>MSSEY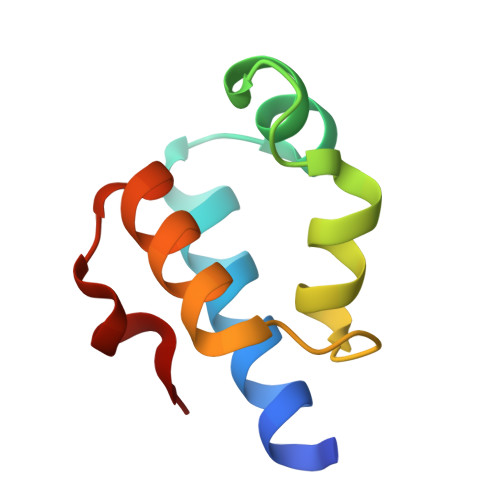AKQLGAKLRAIRTQQGLSLHGVEEKSQGRWKAVVVGSYERGDRAVTVQRLAELADFYGVPVQELLP[3x]> TIAPITGTIKRRVIMDIVLGFSLGG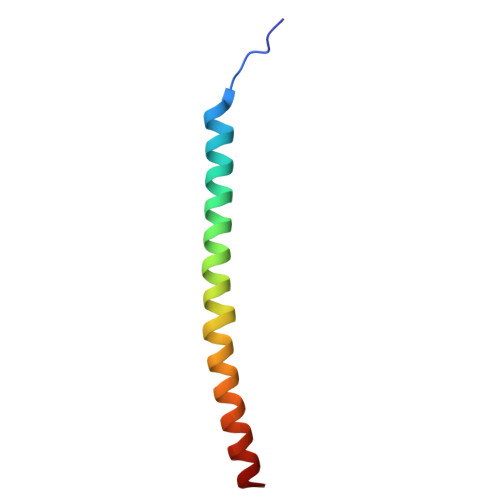VMASYWWWGFHMDKINKREKFYAELAERKK> MAAQNEQRPERIKTTPYLEGDVLSSDSGPLLSVFALQEIMQKVRQVQADYMTATREVDFTVPDVQKILDDIKALAAEQVYKIVKVPSISFRHIVMQSRDRVLRVDTYYEEMSQVGDVITEDEPEKFYSTIIKKVRFIRGKGSFILHDIPTRDHRGMEVAEPEVLGVEFKNVLPVLTAEHRAMIQNALDGSIIENGNVATRDVDVFIGACSEPVYRIYNRLQGYIEAVQLQELRNSIGWLERLGHRKRITYSQEVLTDFRRQDTIWVLALQLPVNPQVVWDVPRSSIANLIMNIATCLPTGEYIAPNPRISSITLTQRITTTGPFAILTGSTPTAQQLNDVRKIYLALMFPGQIILDLKIDPGERMDPAVRMVAGVVGHLLFTAGGRFTNLTQNMARQLDIALNDYLLYMYNTRVQVNYGPTGEPLDFQIGRNQYDCNVFRADFATGTGYNGWATIDVEYREPAPYVHAQRYIRYCGIDSRELINPTTYGIGMTYHCYNEMLRMLVAAGKDSEAAYFRSMLPFHMVRFARINQIINEDLHSVFSLPDDMFNA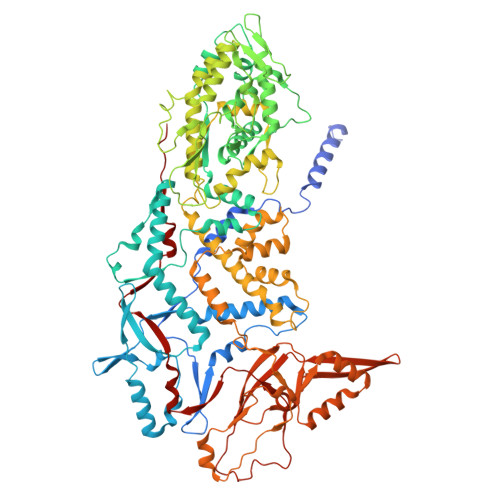LLPDLIAGAHQNADPVVLDVSWISLWFAFNRSFEPTHRNEMLEVAPLIESVYASELSVMKVDMRHLSLMQRRFPDVLIQARPSHFWKAVLNDSPEAVKAVMNLSHSHNFINIRDMMRWVMLPSLQPSLKLALEEEAWAAANDFEDLMLTDQVYMHRDMLPEPRLDDIERFRQEGFYYTNMLEAPPEIDRVVQYTYEIARLQANMGQFRAALRRIMDDDDWVRFGGVLRTVRVKFYDARPPDDVLQGLPFSYDTNERGGLAYATIKYATETTIFYLIYNVEFSNTPDSLVLINPTYTMTKVFINKRIVERVRVGQILAVLNRRFVAYKGKMRIMDITQSLKMGTKLAAPTV However, for these theories to be broadly applicable, they need to be demonstrated for large and multimeric enzymes that catalyze complicated reactions. The enzyme used in this study is a type II DNA topoisomerase (Top2) from African swine fever virus (Asfv), a dimeric multi-subdomain enzyme (271 kDa) that catalyzes multistep reactions to modulate DNA topology. AsfvTop2 has been found to be involved in the early stage of viral gene replication, and also detected at the intermediate and late stages of infection. The domain composition of AsfvTop2 resembles that of the canonical Type IIA DNA topoisomerases (Top2), including the well-studied eukaryotic counterparts, which form homodimers. The catalytic process not only involves well-coordinated changes in protein quaternary structures to allow timely opening and closing of the N-, DNA-, and C-gates, but also ATP binding and sequential hydrolysis that relate the dimerization and catalytic activity of the ATPase domain to the mechanistic steps of the cycle.

We first performed the cryo-EM reconstruction of the full-length apo-AsfvTop2 without DNA or nucleotide. Furthermore, these primary conformational states are each sub-classified into two conformers, a and b, exhibiting local differences. The distribution of the three primary co-existing apo-conformers is approximately 1:4:2. Even though such differences are modest energetically, they do suggest that the closed state II is the most stable state, followed by the C-gate open state III and then the open state I. These thermodynamic properties are reflected in their structural properties described in the following sections. Conformers Ia/Ib were aligned globally with two apo-yeast Top2 structures. The results from the preceding section suggest that, even though the global conformation of apo-IIa is very similar to that of EDI-1, binding of DNA/inhibitor still induces small subdomain reorientations (Supplementary Movie 3: DNA-induced subdomain reorientation of AsfvTop2), yet coupled with substantial catalytically relevant conformational changes locally. On the other hand, as shown in Fig. 4f, the three ß-HPs and the catalytic Y800 in apo-Ia are farther away, relative to the corresponding moieties in apo-IIa, from the catalytically relevant positions in EDI-1, suggesting that it is less feasible for apo-I to bind the DNA substrate and undergo functionally relevant conformational changes.

>MEAFEISDFKEHAKKKSMWAGALNKVTISGLMGVFTEDEDLMALPIHRDHCPALLKIFDELIVNATDHERACHSKTKKVTYIKISFDKGVFSCENDGPGIPIAKHEQASLIAKRDVYVPEVASCFFLAGTNINKAKDCIKGGTNGVGLKLAMVHSQWAILTTADGAQKYVQQINQRLDIIEPPTITPSREMFTRIELMPVYQELGYAEPLSETEQADLSAWIYLRACQCAAYVGKGTTIYYNDKPCRTGSVMALAKMYTLLSAPNSTIHTATIKADAKPYSLHPLQVAAVVSPKFKKFEHVSIINGVNCVKGEHVTFLKKTINEMVIKKFQQTIKDKNRKTTLRDSCSNIFVVIVGSIPGIEWTGQRKDELSIAENVFKTHYSIPSSFLTSMTRSIVDILLQSISKKDNHKQVDVDKYTRARNAGGKRAQDCMLLAAEGDSALSLLRTGLTLGKSNPSGPSFDFCGMISLGGVIMNACKKVTNITTDSGETIMVRNEQLTNNKVLQGIVQVLGLDFNCHYKTQEERAKLRYGCIVACVDQDLDGCGKILGLLLAYFHLFWPQLIIHGFVKRLLTPLIRVYEKGKTMPVEFYYEQEFDAWAKKQTSLVNHTVKYYKGLAAHDTHEVKSMFKHFDNMVYTFTLDDSAKELFHIYFGGESELRKRELCTGVVPLTETQTQSIHSVRRIPCSLHLQVDTKAYKLDAIERQIPNFLDGMTRARRKILAGGVKCFASNNRERKVFQFGGYVADHMFYHHGDMSLNTSIIKAAQYYPGSSHLYPVFIGIGSFGSRHLGGKDAGSPRYISVQLASEFIKTMFPAEDSWLLPYVFEDGQRAEPEYYVPVLPLAIMEYGANPSEGWKYTTWARQLEDILALVRAYVDKDNPKHELLHYAIKHKITILPLRPSNYNFKGHLKRFGQYYYSYGTYDISEQRNIITITELPLRVPTVAYIESIKKSSNRMTFIEEIIDYSSSETIEILVKLKPNSLNRIVEEFKETEEQDSIENFLRLRNCLHSHLNFVKPKGGIIEFNSYYEILYAWLPYRRELYQKRLMREHAVLKLRIIMETAIVRYINESAELNLSHYEDEKEASRILSEHGFPPLNHTLIISPEFASIEELNQKALQGCYTYILSLQARELLIAAKTRRVEKIKKMQARLDKVEQLLQESPFPGASVWLEEIDAVEKAIIKGRNTQWKFHHHHHH[2x]> MAGAIASRMSFSSLKRKQPKTFTVRIVTMDAEMEFNCEMKWKGKDLFDLVCRTLGLRETWFFGLQYTIKDTVAWLKMDKKVLDHDVSKEEPVTFHFLAKFYPENAEEELVQEITQHLFFLQVKKQILDEKIYCPPEASVLLASYAVQAKYGDYDPSVHKRGFLAQEELLPKRVINLYQMTPEMWEERITVWYAEHRGRARDEAEMEYLKIAQDLEMYGVNYFAIRNKK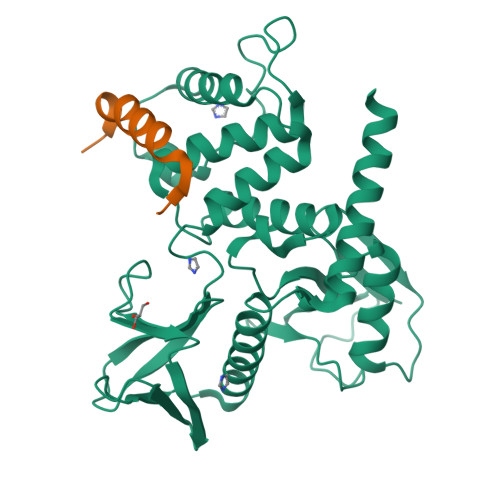GTELLLGVDALGLHIYDPENRLTPKISFPWNEIRNISYSDKEFTIKPLDKKIDVFKFNSSKLRVNKLILQLCIENHDLFMRRRKADSLEVQQMKAQAREEKARKQMERQRL;> PKFGTHHKALQEIRNSLLPFANE> RSHHHHHHGCLTQLYENAFFRGGDVASMYTPNAQYCQMRCTFHPRCLLFSFLPASSINDMEKRFGCFLKDSVTGTLPKVHRTGAVSGHSLKQCGHQISACHRDIYKGVDMRGVNFNVSKVSSVEECQKRCTNNIRCQFFSYATQTFHKAEYRNNCLLKYSPGGTPTAIKVLSNVESGFSLKPCALSEIGCHMNIFQHLAFSDVDVARVLTPDAFVCRTICTYHPNCLFFTFYTNVWKIESQRNVCLLKTSESGTPSSSTPQENTISGYSLLTCKRTLPEPCHSKIYPGVDFGGEELNVTFVKGVNVC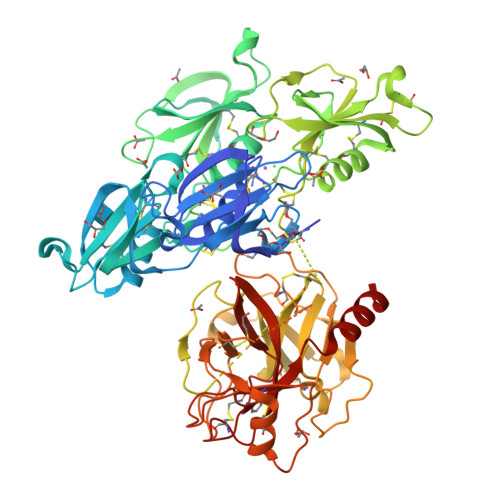QETCTKMIRCQFFTYSLLPEDCKAEACKCFLRLSMDGSPTRIAYGTQGSSGYSLRLCNTGDNSVCTTKTSTRIVGGTQSSWGEWPWQVSLQVKLTAQRHLCGGSLIGHQWVLTAAHCFDGLPLQDVWRIYSGILQLSDITKDTPFSQIKEIIIHQNYKVSEGNHDIALIKLQAPLQYTEFQKPICLPSKGDTSTIYTNCWVTGWGFSAEAGEIQNILQKVNIPLVTNEECQKRYQDYKITQRMVCAGYKEGGKDACKGDAGGPLVCKHNGMWRLVGITSWGEGCARREQPGVYTKVAEYMDWILEKTQSSDGKAQMQSPA> RNIIADKYDEASVLFADIVGFTERASSTAPADLVRFLDRLYSAFDELVDQ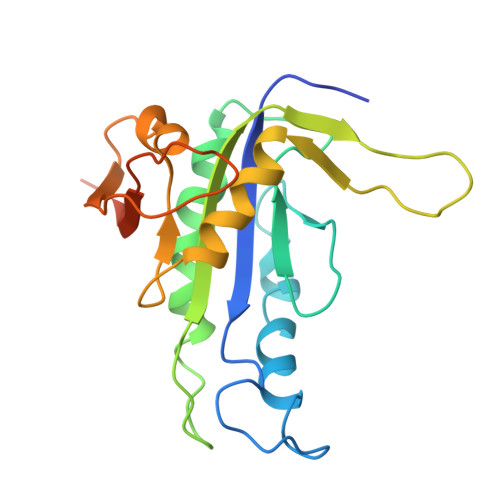HGLEKIEVSGDSYMVVSGVPRPRPDHTQALADFALDMTNVAAQLKDPRGNPVPLRVGLATGPVVAGVVGSRRFRYCVWGDAVNVASRMESTDSVGQIQVPDEVYERLKDDFVLRERGHINVKGKGVMRTWYLIGRKVAADPGEVRGAEPRTAGV>NEIVVYSARADELLKPIAEAYQQKTGTKVTVVSDKAGPLMERLKAEGKNTQADVLITVDGGNLWQATQAGVLRPINSSVLKSNIPSHLRDPKNHWFGLSVRARTIFYNPNKVNPSELSTYADLADPKWKGRLCLRTSNNVYNQSLVATMIANHGQATTDRVVKGWVANLAAAPFANDTALLEAIDAGRCDVGIANTYYYGRLLNSKPQVANNVKVFFANQAGKGTHVNVSGAGVVKHSDNPAEAQKFIEWLSSNEAQRLYADRNFEYPANIQV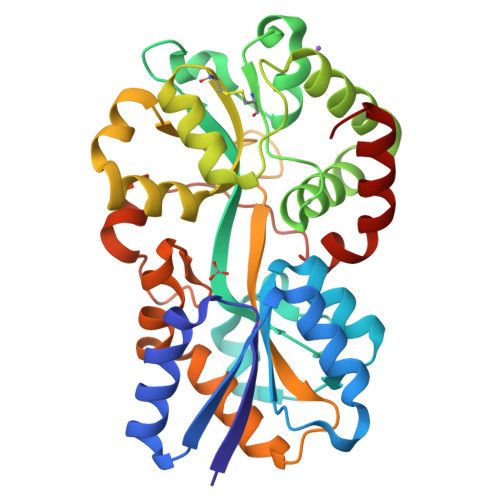TPTPAVARWGRFKQDFINVSVAGQNQQKAIMTMKRAGYK[4x]> MVFKKVLLTGTSEESFTAAADDAIDRAEDTLDNVVWAEVVDQGVE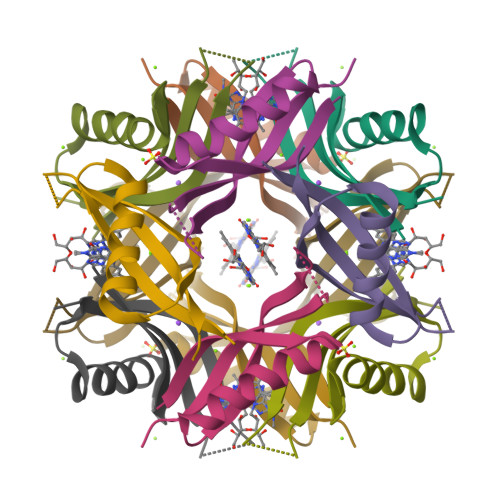IGAVEERTYQTEVQVAFELDGSQ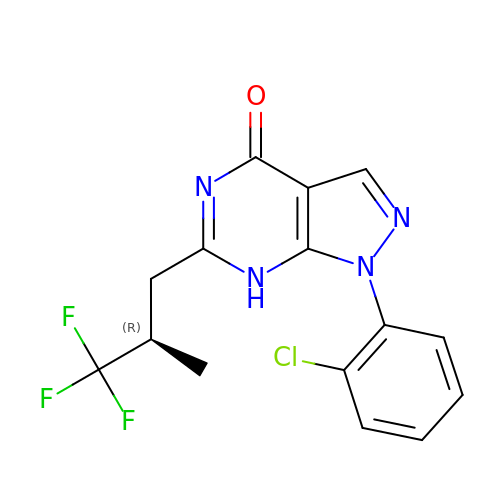1-(2-chlorophenyl)-6-[(2R)-3,3,3-trifluoro-2-methylpropyl]-1,7-dihydro-4H-pyrazolo[3,4-d]pyrimidin-4-one | C15 H12 Cl F3 N4 O | FFPXPXOAFQCNBS-MRVPVSSYSA-N> MEGLAGYVYKAASEGKVLTLAALLLNRSESDIRYLLGYVSQQGGQRSTPLIIAARNGHAKVVRLLLEHYRVQTQQTGTVRFDGYVIDGATALWCAAGAGHFEVVKLLVSHGANVNHTTVTNSTPLRAACFDGRLDIVKYLVENNANISIANKYDNTCLMIAAYKGHTDVVRYLLEQRADPNAKAHCGATALHFAAEAGHIDIVKELIKWRAAIVVNGHGMTPLKVAAESCKADVVELLLSHADCDRRSRIEALELLGASFANDRENYDIIKTYHYLYLAMLERFQDGDNILEKEVLPPIHAYGNRTECRNPQELESIRQDRDALHMEGLIVRERILGADNIDVSHPIIYRGAVYADNMEFEQCIKLWLHALHLRQKGNRNTHKDLLRFAQVFSQMIHLNETVKAPDIECVLRCSVLEIEQSM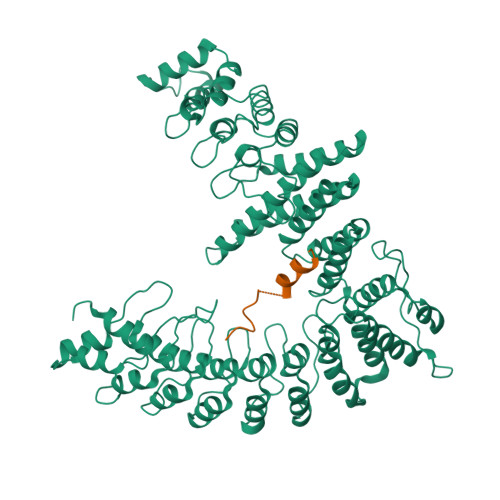NRVKNISDADVHNAMDNYECNLYTFLYLVCISTKTQCSEEDQCKINKQIYNLIHLDPRTREGFTLLHLAVNSNTPVDDFHTNDVCSFPNALVTKLLLDCGAEVNAVDNEGNSALHIIVQYNRPISDFLTLHSIIISLVEAGAHTDMTNKQNKTPLDKSTTGVSEILLKTQMKMSLKCLAARAVRANDINYQDQIPRTLEEFVGFH;> GGGSGGGSKFADHLHKFHENDNGAAAGDLWQ(2~{E})-5-methoxy-2-[[1-(phenylmethyl)piperidin-4-yl]methylidene]-3~{H}-inden-1-one | C23 H25 N O2 | 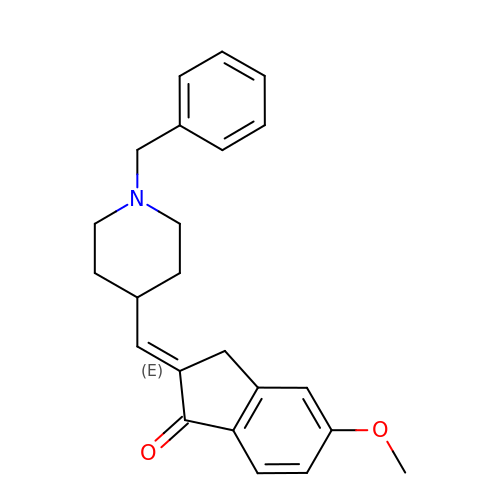CNIWTTNRVIMZIP-DEDYPNTBSA-N> PISPIETVPVKLKPGMDGPKVKQWPLTEEKIKALVEICTEMEKEGKISKIGPENPYNTPVFAIKKKDGTKWRKLVDFRELNKKTQDFWEVQLGIPHPAGLKKKKSVTVLDVGDAYFSVPLDEDFRKYTAFTIPSINNETPGIRYQYNVLPQGWKGSPAIFQSSMTKILEPFRKQNPDIVIYQYMDDLYVGSDLEIGQ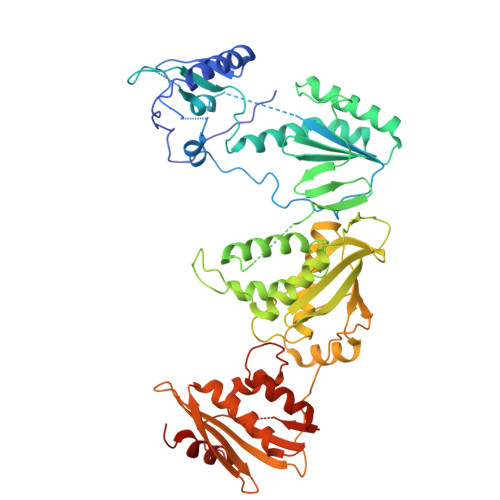HRTKIEELRQHLLRWGLTTPDKKHQKEPPFLWMGYELHPDKWTVQPIVLPEKDSWTVNDIQKLVGKLNWASQIYPGIKVRQLCKLLRGTKALTEVIPLTEEAELELAENREILKEPVHGVYYDPSKDLIAEIQKQGQGQWTYQIYQEPFKNLKTGKYARMRGAHTNDVKQLTEAVQKITTESIVIWGKTPKFKLPIQKETWETWWTEYWQATWVPEWEFVNTPPLVKLWYQLEKEPIVGAETFYVDGAASRETKLGKAGYVTNKGRQKVVTLTDTTNQKTELQAIHLALQDSGLEVNIVTASQYALGIIQAQPDQSESELVNQIIEQLIKKEKVYLAWVPAHKGIGGNEQVDKLVSAGIRKIL>MPKRIVYNISSDFQLKSLLGEGAYGVVCSATHKPTGEIVAIKKIEPFDKPLFALRTLREIKILKHFKHENIITIFNIQRPDSFENFNEVYIIQELMQTDL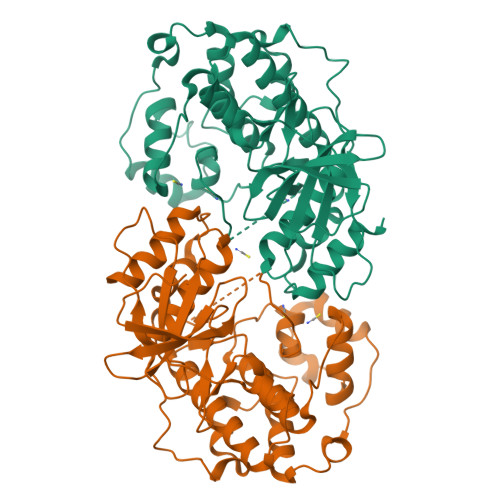HRVISTQMLSDDHIQYFIYQTLRAVKVLHGSNVIHRDLKPSNLLINSNCDLKVCDFGLARIIDESAADNSEPTGQQSGMVEFVATRWYRAPEVMLTSAKYSRAMDVWSCGCILAELFLRRPIFPGRDYRHQLLLIFGIIGTPHSDNDLRCIESPRAREYIKSLPMYPAAPLEKMFPRVNPKGIDLLQRMLVFDPAKRITAKEALEHPYLQTYHDPNDEPEGEPIPPSFFEFDHYKEALTTKDLKKLIWNEIFS[2x]>[2x]TNLVAEPFAKLEQDFGGSIGVYAMDTGSGATVSYRAEERFPLCSSYKGFLAAAVLARSQQQAGLLDTPIRYGKNALVPWSPISEKYLTTGMTVAELSAAAVQYSDNAAANLLLKELGGPAGLTAFMRSIGDTTFRLDRWELELNSAIPGDARDTSSPRAVTESLQKLTLGSALAAPQRQQFVDWLKGNTTGNHRIRAAVPADWAV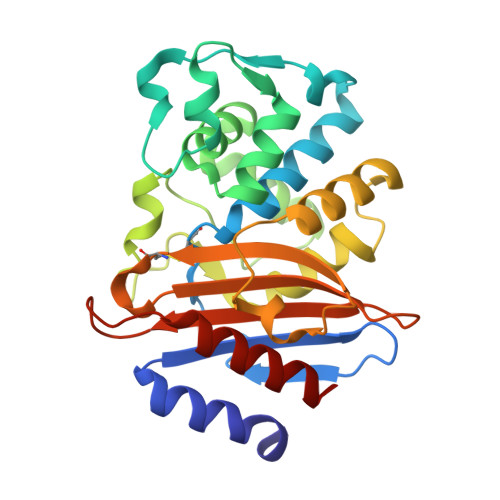GDKTGTCGVYGTANDYAVVWPTGRAPIVLAVYTRAPNKDDKHSEAVIAAAARLALEGLG> MLKQVEIFTDGSCLGNPGPGGYGAILRYRGREKTFSAGYTRTTNNRMELMAAIVALEALKEHCEVILSTDSQYVRQGITQWIHNWKKRGWKTADKKPVKNVDLWQRLDAALGQHQIKWE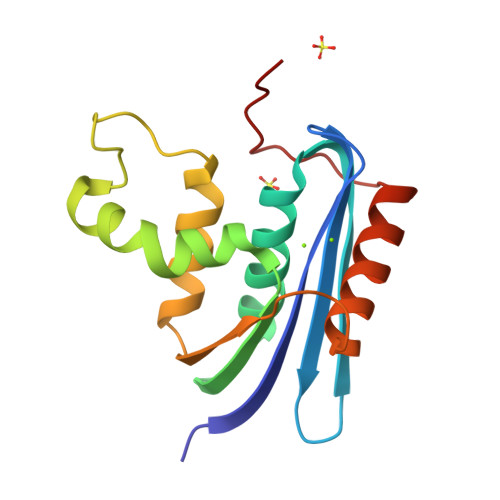WVKGHAGHPENERCDELARAAAMNPTLEDTGYQVEV> GLPGSMNDRADFVVPDITTRKNVGLSHDANDFTLPQPLDRYSAEDHATWATLYQRQCKL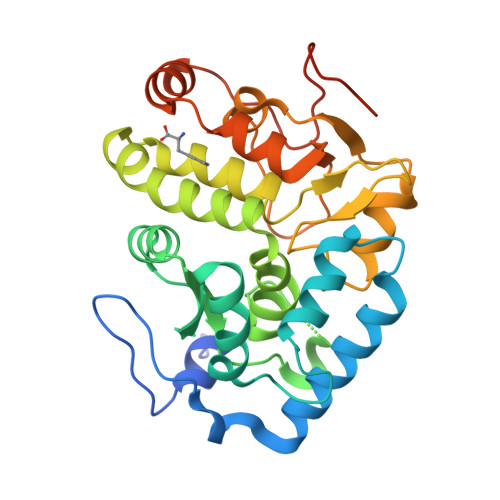LPGRACDEFLEGLERLEVDADRVPDFNKLNEKLMAATGWKIVAVPGLIPDDVFFEHLANRRFPVTWWLREPHQLDYLQEPDVFHDLFGHVPLLINPVFADYLEAYGKGGVKAKALGALPMLARLYWYTVEFGLINTPAGMRIYGAGILPSKSESIYCLDSASPNRVGFDLMRIMNTRYRIDTFQKTYFVIDSFKQLFDATAPDFAPLYLQLADAQPWGAGDIAPDDLVLNAGDHQGWADTEDV N-[1-(5-{[(4-fluorophenyl)methyl]sulfanyl}-4-methyl-4H-1,2,4-triazol-3-yl)ethyl]-2-(trifluoromethyl)benzamide 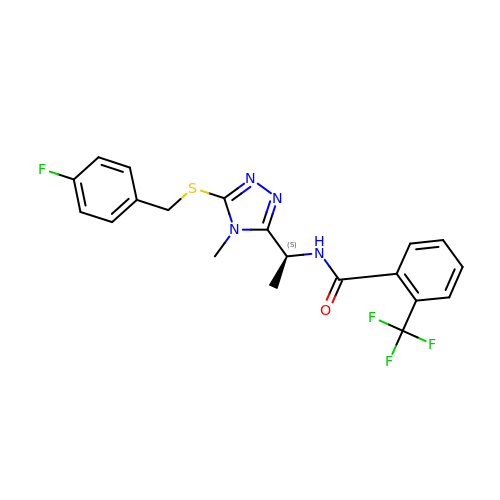| C20 H18 F4 N4 O S | WAMHSAKMZVUOGV-LBPRGKRZSA-N>[8x]MDKFRVQGPTRLQGEVTISGAKNAALPILFAALLAEEPVEIQNVPKLKDIDTTMKLLTQLGTKVERDGSVWIDASNVNNFSAPYDLVKTMRASIW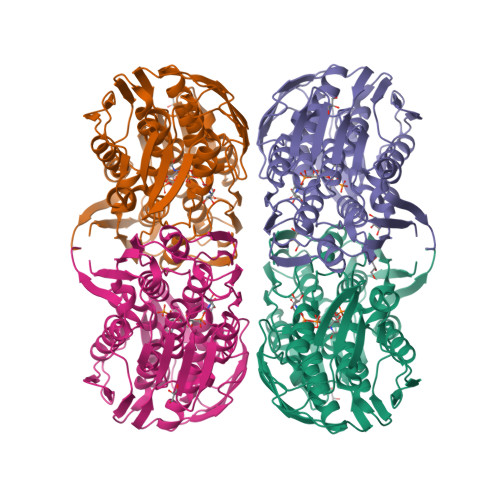ALGPLVARFGQGQVSLPGGSAIGARPVDLHIFGLEKLGAEIKLEEGYVKASVNGRLKGAHIVMDKVSVGATVTIMSAATLAEGTTIIENAAREPEIVDTANFLVALGAKISGQGTDRITIEGVERLGGGVYRVLPDRIETGTFLVAAAISGGKIVCRNAQPDTLDAVLAKLREAGADIETGEDWISLDMHGKRPKAVTVRTAPHPAFPTDMQAQFTLLNLVAEGTGVITETIFENRFMHVPELIRMGAHAEIESNTVICHGVEKLSGAQVMATDLRASASLVLAGCIAEGTTVVDRIYHIDRGYERIEDKLRALGANIERVKGE> MKDLLKFLKAQTKTEEFDAIKIALASPDMIRSWSFGEVKKPETINYRTFKPERDGLFCARIFGPVKDYECLCGKYKRLKHRGVICEKCGVEVTQTKVRRERMGHIELASPTAHIWFLKSLPSRIGLLLDMPLRDIERVLYFESYVVIEGGMTNLERQQILTEEQYLDALEEFGDEFDAKMGAEAIQALLKSMDLEQECEQLREELNETNSETKRKKLTKRIKLLEAFVQSGNKPEWMILTVLPVLPPDLRPLVPLDGGRFATSDLNDLYRRVINRNNRLKRLLDLAAPDIIVRNEKRMLQEAVDALLDNGRRGRAITGSNKRPLKSLADMIKGKQGRFRQNLLGKRVDYSGRSVITVGPYLRLHQCGLPKKMALELFKPFIYGKLELRGLATTIKAAKKMVEREEAVVWDILDEVIREHPVLLNRAPTLHRLGIQAFEPVLIEGKAIQLHPLVCAAYNADFDGDQMAVHVPLTLEAQLEARALMMSTNNILSPANGEPIIVPSQDVVLGLYYMTRDCVNAKGEGMVLTGPKEAERLYRSGLASLHARVKVRITEYEKDANGELVAKTSLKDTTVGRAILWMIVPKGLPYSIVNQALGKKAISKMLNTCYRILGLKPTVIFADQIMYTGFAYAARSGASVGIDDMVIPEKKHEIISEAEAEVAEIQEQFQSGLVTAGERYNKVIDIWAAANDRVSKAMMDNLQTETVINRDGQEEKQVSFNSIYMMADSGARGSAAQIRQLAGMRGLMAKPDGSIIETPITANFREGLNVLQYFISTHGARKGLADTALKTANSGYLTRRLVDVAQDLVVTEDDCGTHEGIMMTPVIEGGDVKEPLRDRVLGRVTAEDVLKPGTADILVPRNTLLHEQWCDLLEENSVDAVKVRSVVSCDTDFGVCAHCYGRDLARGHIINKGEAIGVIAAQSIGEPGTQLTMRTFHIGGAASRAAAESSIQVKNKGSIKLSNVKSVVNSSGKLVITSRNTELKLIDEFGRTKESYKVPYGAVLAKGDGEQVAGGETVANWDPHTMPVITEVSGFVRFTDMIDGQTITRQTDELTGLSSLVVLDSAERTAGGKDLRPALKIVDAQGNDVLIPGTDMPAQYFLPGKAIVQLEDGVQISSGDTLARIPQESGGTKDITGGLPRVADLFEARRPKEPAILAEISGIVSFGKETKGKRRLVITPVDGSDPYEEMIPKWRQLNVFEGERVERGDVISDGPEAPHDILRLRGVHAVTRYIVNEVQDVYRLQGVKINDKHIEVIVRQMLRKATIVNAGSSDFLEGEQVEYSRVKIANRELEANGKVGATYSRDLLGITKASLATESFISAASFQETTRVLTEAAVAGKRDELRGLKENVIVGRLIPAGTGYAYHQDRMRRRAAGEAPAAPQVTAE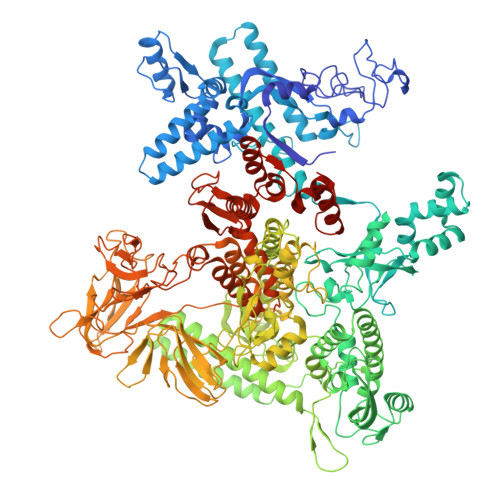DASASLAELLNAGLGGSDN> MQTKLTIWCSEKQVDILQKLGEEFKAKYGIPVEVQYVDFGSIKSKFLTAAPQGQGADIIVGAHDWVGELAVNGLIEPIPNFSDLKNFYDTALKAFSYGGKLYGVPYAMEAVALIYNKDYVDSVPKTMDELIEKAKQIDEEYGGEVRGFIYDVANFYFSAPFILGYGGYVFKETPQGLDVTDIGLANEGAVKGAKLIKRMIDEGVLTPGDNYGTMDSMFKEGLAAMIINGLWAIKSYKDAGINYGVAPIPELEPGVPAKPFVGVQGFMINAKSPNKVIAMEFLTNFIARKETMYKIYLADPRLPARKDVLELVKDNPDVVAFTQSASMGTPMPNVPEMAPVWSAMGDALSIIINGQASVEDALKEAVEKIKAQIEKGSHHHHHH

Periplasmic binding proteins (PBPs) are the ligand-binding components of ATP-binding cassette (ABC) transporters and are sometimes associated with chemotaxis systems. Members of the PBP superfamily mediate the uptake and transmembrane transport of a diversity of metabolically important solutes in bacteria, such as carbohydrates, ions, amino acids, and polyamines, to name a few. Despite the wide variation in PBP ligand size and chemical functionality the two domain PBPs have a conserved αβ-fold, with each domain encompassing a central β-stranded core that is sandwiched between surrounding α-helices. Ligand binding at the interdomain interface induces a hinge-bending motion in which the two solvent exposed polar interfaces of each domain close down on and envelop ligands in a largely desolvated binding site reminiscent of the protein interior.

Here we report the first neutron crystal structure of a PBP, namely a maltodextrin-binding protein (MBP) from a cluster of three related proteins found in Thermotoga maritima (tmMBP). The room temperature X-ray crystal structure of the tmMBP complexed with maltotetraose was determined at 1.70 Å with an Rwork/Rfree of 14.1/17.5%. The final room temperature neutron structure was determined to a resolution of 2.10 Å and refined to an Rwork/Rfree of 24.3/27.3%. The neutron structure enabled the modelling of deuterium atoms at exchangeable sites on the protein and the bound ligand, as well as deuterium atoms on solvent water molecules. Importantly, the neutron structure also resolves the position and orientation of D2O solvent molecules within the substrate binding cavity, which were previously inferred to provide hydrogen bonding interactions in the earlier cryogenic X-ray model. The tmMBP binding site uses a network of polar amino acids to satisfy the hydrogen bonding potential of many of the maltotetraose hydroxyl groups. A total of 8 specific hydrogen bonds, defined here as mediated either through direct protein/carbohydrate hydrogen bonds or through directly-bound water molecules, are observed for the first two sugar rings (ring 1/R1 and ring 2/R2). A total of 4 specific hydrogen bonds are formed with the remaining two rings (ring 3/R3 and ring 4/R4). The differential hydrogen bonding pattern of the R1/R2 and R3/R4 subsites suggests the tmMBP has a bipartite binding site. The water molecules bound in the specificity subsite are responsible for forming 3 of 8 hydrogen bonds and are thus important in binding of saccharides in tmMBP.>MSVAYNPQTKQFHLRAGKASYVMQLFRSGYLAHVYWGKAVRDVRGARAFPRLDRAFSPNPDPSDRTFSLDTLLQEYPAYGNTDFRAPAYQVQLENGSTVTDLRYKTHRIYKGKPRLNGLPATYVEHEQEAETLEIVLGDALIGLEVTLQYTAYEKWNVITRSARFENKGGERLKLLRALSMSVDFPTADYDWIHLPGAWGRERWIERRPLVTGVQAAESRRGASSHQQNPFIALVAKNADEHQGEVYGFSFVYSGNFLAQIEVDQFGTARVSMGINPFDFTWLLQPGESFQTPEVVMVYSDQGLNGMSQTYHELYRTRLARGAFRDRERPILINNWEATYFDFNEEKIVNIARTAAELGIELVVLDDGWFGERDDDRRSLGDWIVNRRKLPNGLDGLAKQVNELGLQFGLWVEPEMVSPNSELYRKHPDWCLHVPNRPRSEGRNQLVLDYSREDVCDYIIETISNVLASAPITYVKWDMNRHMTEIGSSALPPERQRETAHRYMLGLYRVMDEITSRFPHILFESCSGGGGRFDPGMLYYMPQTWTSDNTDAVSRLKIQYGTSLVYPISAMGAHVSAVPNHQVGRVASLKTRGHVAMSGNFGYELDITKLTETEKQMMKQQVAFYKDVRRLVQFGTFYRLLSPFEGNEAAWMFVSADRSEALVAYFRVLAEANAPLSYLRLKGLDSNQDYEIEGLGVYGGDELMYA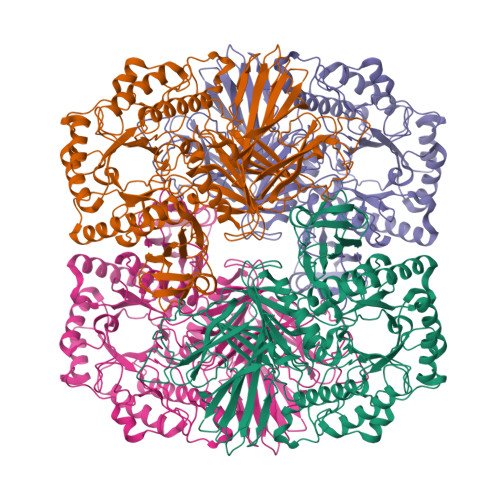GVALPYRSSDFISMMWRLKAVQQ[4x]(5S)-2-amino-3-methyl-5-[3-(pyridin-3-yl)phenyl]-5-(thiophen-3-yl)-3,5-dihydro-4H-imidazol-4-one | C19 H16 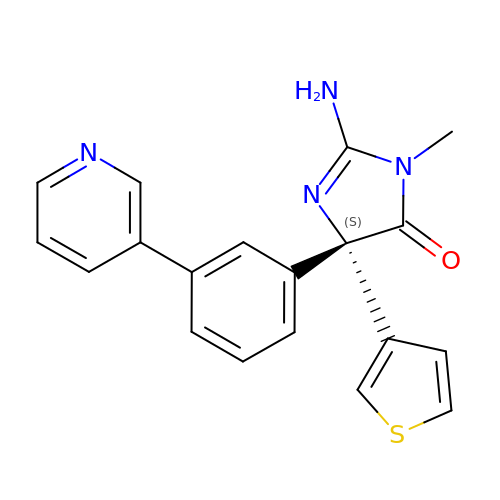N4 O S | AOGBXAFIKRFUPJ-IBGZPJMESA-N>[2x]AARQMEALNRGLVAVKTDGGIFVSWRFLGTENASVLFNVYRDGQKLNAAPVKTTNYVDKNGSAGSTYTVRAVVNGTEQPASEKASVWAQPYHSVPLDKPAGGTTPKGESYTYSANDASVGDVDGDGQYELILKWDPSNSKDNSQDGYTGDVLIDAYKLDGTKLWRINLGKNIRAGAHYTQFMVYDLDGDGKAEVAMKTADGTKDGTGKVIGNANADYRNEQGRVLSGPEYLTVFQGSTGKELVTANFEPARGNVSDWGDSYGNRVDRFLAGIAYLDGQRPSLIMTRGYYAKTMLVAYNFRDGKLSKLWTLDSSKSGNEAFAGQGNHNLSIADVDGDGKDEIIFGSMAVDHDGKGMYSTGLGHGDALHTGDLDPGRPGLEVFQVHEDKNAKYGLSFRDAATGKILWGVYAGKDVGRGMAADIDPRYPGQEVWANGSLYSAKGVKIGSGVPSSTNFGIWWDGDLLREQLDSNRIDKWDYQNGVSKNMLTASGAA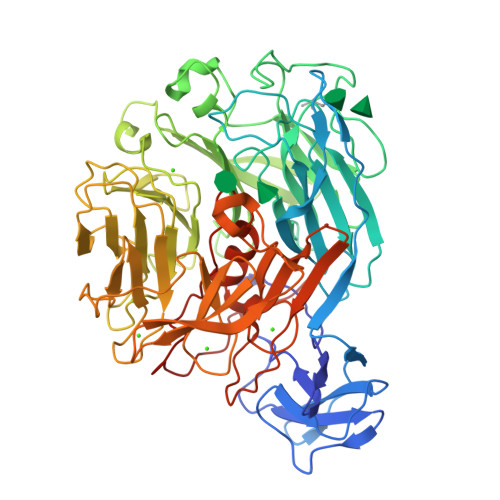ANNGTKATPTLQADLLGDWREEVVWRTEDSSALRIYTTTIPTEHRLYTLMHDPVYRLGIAWQNIAYNQPPHTSFFLGDGMAEQPKPNMYTPLEHHHHHH> HHHHHHMRVLGLNGWPRDFHDASAALLVDGRIAAFAEEERFTRKKHGYNTAPVQAAAFCLAQAGLTVDDLDAVAFGWDLPAMYRERLGGWPHSDSEALDILLPRDVFPRRTDPPLHFVQHHLAHAASAYYFSGEDRGAVLIVDGQGEEECVTLAHAEGGKITVLDTVPGAWSLGFFYEHVSEYTGLGGDNPGKLMGLAAHGTTVDETLSAFAFDSDGYRLNLIDPQARDPEDWDEYSVTERAWFAHLERIYRLPPNEFVRRYDPAKGRVVRDTRRDPYEYRDLAATAQAALERAVFGLADSVLARTGERTLFVAGGVGLNATMNGKLLTRSTVDKMFVPPVASDIGVSLGAAAAVAV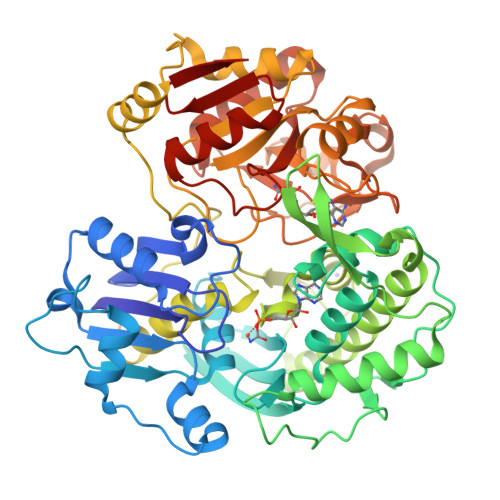ELGDRIAPMGDTAAWGPEFSPDQVRAALDRTGLAYREPANLEREVAALIASGKVVGWAQGRGEVGPRALGQRSLLGSAHSPTMRDHINLRVKDREWWRPFAPSMLRSVSDQVLEVDADFPYMIMTTKVRAAYAERLPSVVHEDWSTRPQTVTEASNPRYHRMLTELGDLVGDPVCLNTSFNDRGEPIVSSPADALLTFSRLPIDALAVGPYLVTKDLRH4-{1-[2-chloro-6-(trifluoromethyl)benzoyl]-1H-pyrazolo[4,3-b]pyridin-3-yl}-5-fluoro-2-hydroxybenzoic 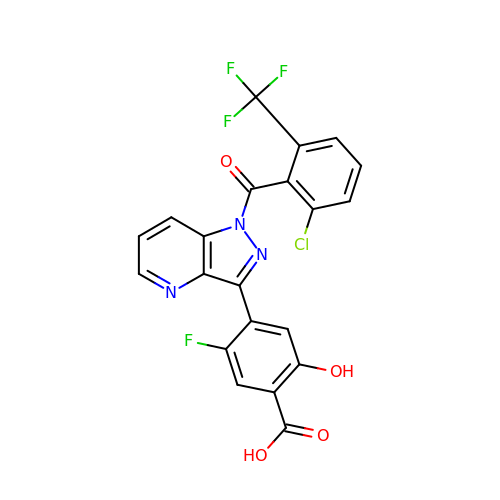acid | C21 H10 Cl F4 N3 O4 | VYMOEMKHCRZWMT-UHFFFAOYSA-N> SMAFKIQLDTLGQLPGLLSIYTQISLLYPVSDSSQYPTIVSTFEQGLKRFSEAVPWVAGQVKAEGISEGNTGTSFIVPFEDVPRVVVKDLRDDPSAPTIEGMRKAGYPMAMFDENIIAPRKTLPIGPGTGPDDPKPVILLQLNFIKGGLILTVNGQHGAMDMVGQDAVIRLLSKACRNDPFTEEEMTAMNLDRKTIVPYLENYTIGPEVDHQIVKADVAGGDAVLTPVSASWAFFTFSPKAMSELKDAATKTLDASTKFVSTDDALSAFIWKSASRVRLERIDGSAPTEFCRAVDARPAMGVSNNYPGLLQNMTYHNSTIGEIANESLGATASRLRSELDPASMRQRTRGLATYLHNNPDKSNVSLTADADPSTSVMLSSWAKVGLWDYDFGLGLGKPETVRRPIFEPVESLMYFMPKKPDGEFCAAL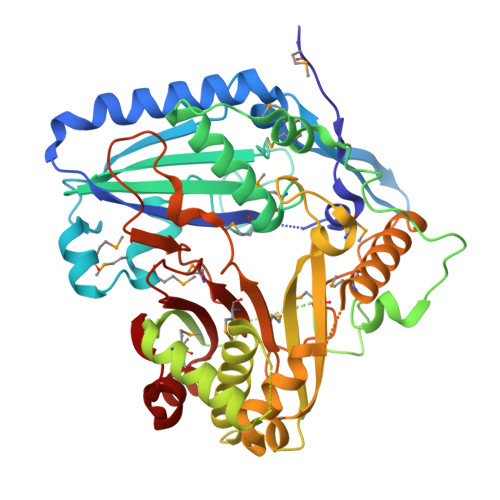SLRDEDMDRLKADKEWTKYAQYVG> MLPLSIEQRRPSRSPEYDQSTLSNYKDFAVLHTDLNLSVSFEKSAISGSVTFQLKKLHEGKNKSDELHLDTSYLDVQEVHIDGSKADFQIEQRKEPLGS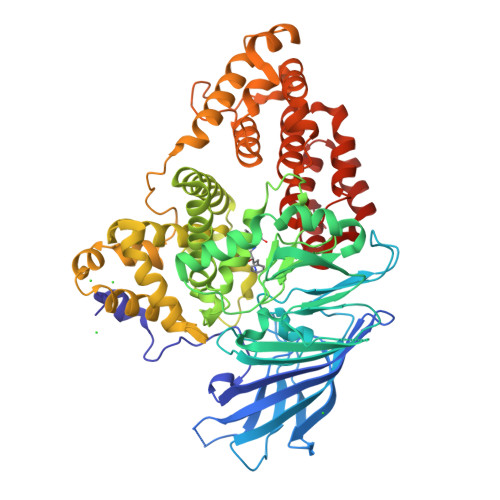RLVINNASCNDNFTLNIQFRTTDKCTALQWLNSKQTKGGKPYVFSQLEAIHARSLFPCFDTPSVKSTFTASIESPLPVVFSGIRIEDTSKDTNIYRFEQKVPIPAYLIGIASGDLSSAPIGPRSTVYTEPFRLKDCQWEFENDVEKFIQTAEKIIFEYEWGTYDILVNVDSYPYGGMESPNMTFATPTLLAHDRSNIDVIAHELAHSWSGNLVTNCSWNHFWLNEGWTVYLERRIIGAIHGEPTRHFSALIGWSDLQNSIDSMKDPERFSTLVQNLNDNTDPDDAFSTVPYEKGFNLLFHLETILGGKAEFDPFIRHYFKKFAKKSLDTFQFLDTLYEFYPEKKEILDSVDWETWLYKPGMPPRPHFITALADNVYQLADKWVEMAQHLKTTEDFRSEFNAIDIKDFNSNQLVLFLETLTQNGHSNKKPKDFDWAKFPVASRALLDIYQDNIVKSQNAEVVFKMFKFQIFAKLQEEYKHLADWLGTVGRMKFVRPGYRLLNSVDRRLALATFDKFKDTYHPICKALVKQDLKL> MEKFVLSLDEGTTSARAIIFDRESNIHGIGQYEFPQHYPRPGWVEHNPEEIWDAQLRAIKDAIQSARIEPNQIAAIGVTNQRETTLVWDK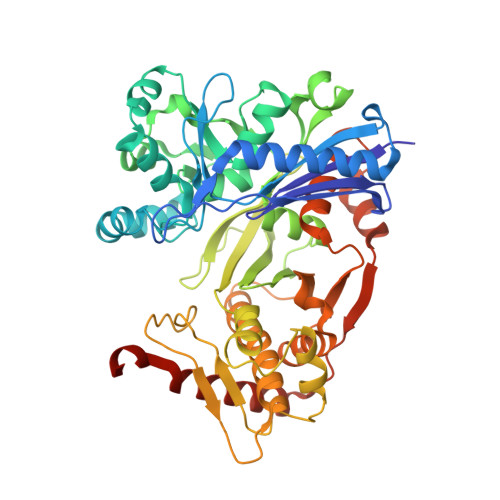DGKPLYNAIVWQCRRTAEMVEEIKREYGTMIKEKTGLVPDAYFSASKLKWLLDNLPGLREKAEKGEVMFGTVDTFLIYRLTGEHVTDYSNASRTMLFNIKKLDWDDELLELFDIPESVLPEVRESSEVYGYTKKELLGAEIPVSGDAGDQQAALFGEAAFEAGMVKATYGTGSFILVNTDEMVLYSDNLLTTIAWGLNGRVSYALEGSIFVTGAAVQWLRDGIKIIKHASETEELATKLESNEGVYFVPAFVGLGAPYWDQFARGIIIGITRGTGREHLARATLEAIAYLTRDVVDEMEKLVQIKELRVDGGATANDFLMQFQADILNRKVIRPVVKETTALGAAYLAGLAVDYWADTREIAELWKAERIFEPKMDEKTRERLYKGWKEAVKRAMGWAKVVDSAKSN> SEFMSQSNRELVVDFLSYKLSQKGYSWSQFSDVEENRTEAPEGTESEAVKQALREAGDEFELRYRRA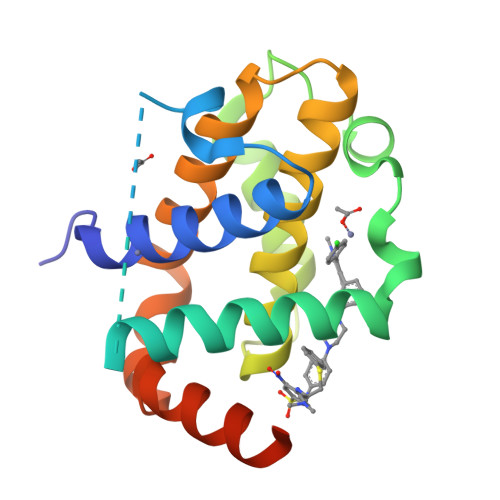FSDLTSQLHITPGTAYQSFEQVVNELFRDGVNWGRIVAFFSFGGALCVESVDKEMQVLVSRIAAWMATYLNDHLEPWIQENGGWDTFVELYGNNAAAESRKGQER> GAPATVTEQGEDITSKKDRGVLKIVKRVGNGEETPLIGDKVYVHYKGALSNGKKEDSSHDRNEPFVFSLGKGQVIKAWDIGVATLKKGEIAHLLIKPEYAYGSAGSLPKIPSNATLFFEIELLDFKGE

Here we used the FK506-binding protein 51 (FKBP51) as a model system to evaluate whether chemically engineered proteins can be trapped in pharmacologically relevant conformations. FKBP51 has emerged as a promising drug target for chronic pain, obesity, and depression. The major challenge in FKBP51 drug development is selectivity toward its closest homologue FKBP52, as the binding pockets of both proteins are very similar, but the biological functions are opposite. Selectivity for FKBP51 can be achieved by targeting a transient conformation characterized by an outward flip of phenylalanine 67 (F67in and F67out).41−45 This conformation is rarely populated in the apo-state of FKBP51,46 but enables high selectivity vs FKBP52.47,48 To stabilize the transient binding pocket of FKBP51 (F67-out), we aimed to lock this conformation precisely by the formation of an intramolecular amide bond (sites displayed in Figure 1B).

Two positions, K58 and K60, were identified as promising anchor points for lactamization to the residue in position 67. This was expected to trap residue 67 in an out-like conformation and stabilize the β2-β3a-loop by a seven (i, i+7) or nine (i, i+9) amino acid macrocycle. Furthermore, for position 60, the size of the macrocycle was finetuned by incorporating ornithine (Orn) or diaminobutyric acid (Dab) as smaller lysine analogues. Protein crystallography of the ligand-bound proteins confirmed the desired 3D structure of the synthesized and refolded proteins FKBP5116–140 F67E/K58 (i, i+9) and F67E/K60Orn (i, i+7). The protein fold, the ligand binding mode, and the conformation of the β3-strand were identical to recombinant FKBP51. Notably, the side chains of F67E/K58 and F67K60 were well resolved, which unambiguously confirmed the desired lactam bridge and its F67-out mimicking conformation. In contrast, for the lactam-bridged variants, fragments resulting from cleavage between F67E/K58, F67E/K60Orn, and F67E/K60Dab are undetectable because the covalent bond formed protects the protein from fragmentation at these sites. Lactamization within the protein was expected to shift the conformational equilibrium toward the F67-out-like conformation. This should result in a higher binding affinity of conformation-specific ligands, as the energetic penalty to adopt the F67-out-like conformation is reduced. When lysine is replaced by the smaller ornithine, up to 39-fold improvement is achieved.> GPLGSMDSSQLHVAIVSSPGMGHLIPVLVLGNRLATHHNIKITILAITTTSSSAETEFLKKTTLTNEEKTIEIIPVPSVDISHLINSSTKIFTQLRLLVREALPKIHSTIASMTHRPDALIVDIFCTQILPIAEEFNISKYTYHPTTAWTLALAIYCQVFDKEIEGEYVELKEPLKIPGCKALRPDDVVDPLLDRSDQQYEEYVKLGKEYTDFDGILINTWEDLEPETINALRYNEKLRLLLKVPVFPIGPLRRKVETTLNDEVIQWLDKQNNESVLFVSFGSGGTLSTKQMTELAWGLELSQQKFVWVVRPPSDGDADSAYLNSAGKDTRDMSEYLPEGFLTRTKDMGLVVPMWANQVEILSHSSVGGFLTHCGWNSTVESLTNGVPMIAWPLHAEQKMNAAMLTEELGVAIRPAVLPTKKLVKREEIQGMVRILMQTKEGKRIKEKAKKLKKSAENALSDGGSSYNSICELVKDIRSR

NbUGT72AY1 is a promiscuous transferase that glycosylates bioactive hydroxycoumarins such as scopoletin and umbelliferone, as well as monolignols involved in lignin formation and various other small molecules. Five distinct GT protein folds have been identified that are capable of GT activity (termed GT-A to GT-E). NbUGT72AY1 adopts a GT-B fold comprised of two distinct N-terminal and C-terminal Rossmann-like domains (shown in cyan and brown in Fig. 2, respectively) of seven and six parallel β-sheets, respectively linked to α-helices, connected by a linker region and an interdomain cleft. The catalytic mechanism of inverting UGT such as NbUGT72AY1 is a direct displacement bimolecular nucleophilic substitution (SN2)-like reaction enabled by an enzymatic base catalyst.

In addition to the apo-form (I), a protein structure was obtained, which crystallized in β-carotene-containing solution (II), differed from the apo-form, and lacked the electron density for the ligand. However, since the addition of apocarotenoids increased the H/D exchange in H124, these effectors reverse the helix-forming effect of scopoletin and the corresponding H2 amino acids should therefore remain flexible. Consistent with this hypothesis, electron density maps derived from crystals grown with β-carotene failed to resolve the secondary structure between Ile42 and Phe53 (complex II). In all NbUGT72AY1 crystals obtained in solutions with retinol or β-carotene, the amino acid sequence between Ser309 and Asp327 (closing loop) is disordered regardless of whether acceptor and/or donor substrates are present (II, VI-IX). Although all the crystals that formed in the presence of 0.5 mM β-carotene and retinol were clearly different from their (apo)carotenoid-free counterparts (I and V versus II and VI, respectively), the effector molecules were not detectable in the electron density map and are invisible in the 3D structure. This may indicate that the effectors bind in a fuzzy way, possibly through poorly directional hydrophobic interactions, leading to multiple positions and orientations in the crystal that are equally likely, or that the effector occupancy of protein molecules in the crystal is too low. In both cases (β-carotene and retinol docked on II and VII, respectively), a majority of the ligand population occupies the hydrophobic acceptor-binding site in the cleft representing the active site, while a smaller number is bound to nonpolar wells on the surface of the protein. The lowest number of interactions (total edges) was calculated for the protein in the presence of β-carotene (II), while the highest number of bonds was obtained after addition of UDP (IV_A and IV_B), which is consistent with the assumption that the carotenoid promotes protein dynamics, while in the product-inhibited complex the mobility of the protein is hindered. (Apo)carotenoids play a role as placeholders.> MSFDPNNPRTITAQTLEGALPVDILLRLNRATGLQMDAAEAHAIVEDARRTLFIGTSLALVNLRRAHDKHLVERQPMFATSDYSSWARPTVGLKRTFCPRPP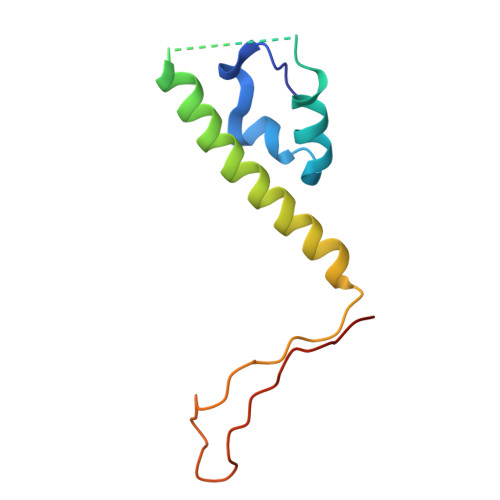P>ACGLVASNLNLKPGECLRVRGEVAADAKSFLLNLGKDDNNLCLHFNPRFNAHGDVNTIVCNSKDAGAWGAEQRESAFPFQPGSVVEVCISFNQTDLTIKLPDGYEFKFPNRLNLEAINYLSAGGDFKIKCVAFE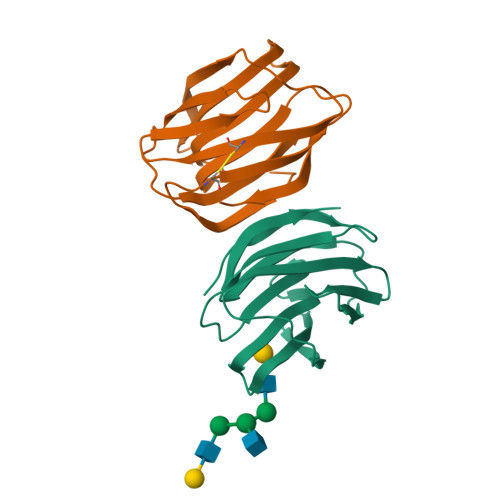[2x]>GMTTATHPNDALFAGEKSFPVLAACEHFAGSEKLIGKAMDLQVEYGPVFDVTCDCEDGAAAGQEREHAEMVARMIASDRNVHGRAGARIHDPSHPAWRQDVDIIVNGAGGRLAYITVPKATNSGQVAEVIRYIGDVAKRAGLDKPVPVHVLIETHGALRDVFQIAELPNIEVLDFGLMDFVSGHHGAIPAAAMRSPGQFEHALLVRAKADMVAAALANGIVPAHNVCLNLKDAEVIASDACRARNEFGFLRMWSIYPAQIQPIVNAMRPDFTEV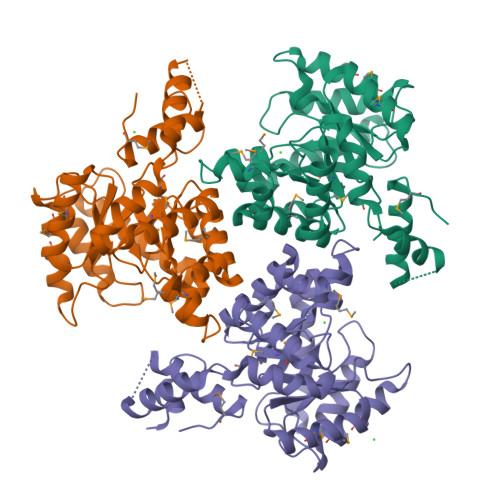EDAAGILVAAQDADWGPIQYKGELHDRATYRYFWEVLQKAKVTGMAVPAEAERRFFVN[6x]> GSSGSSGMMLSLNNLQNIIYNPVIPYVGTIPDQLDPGT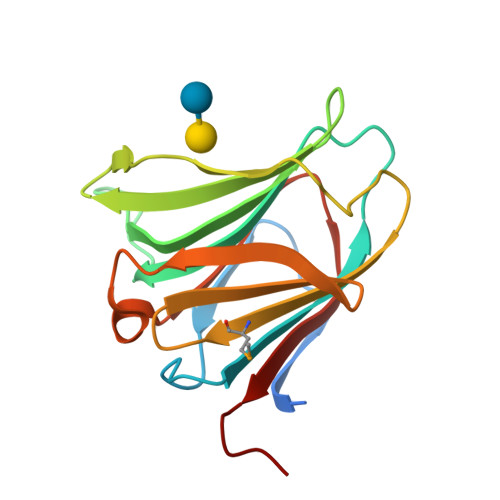LIVICGHVPSDADRFQVDLQNGSSVKPRADVAFHFNPRFKRAGCIVCNTLINEKWGREEITYDTPFKREKSFEIVIMVLKDKFQVAVNGKHTLLYGHRIGPEKIDTLGIYGKVNIHSIGFSGPSSG> QFAKPEDAVKYRQSAATLMASHFGRMTPVVKGQAPYDAAQIKANVEVLKTLSALPWAAFGPGTEGGDARPEIWSDAASFKQKQQAFQDNIVKLSAAADAGDLD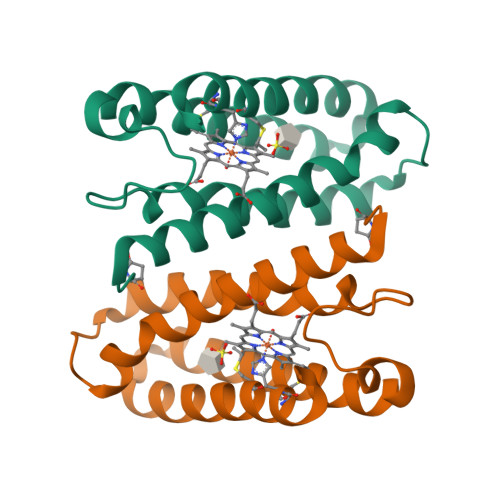KLRAAFGDVGASCKACHDAYRK> TFEYGDGI;> HHHHHHMAIYADNSYSIGNTPLVRLKHFGHNGNVVVKIEGRNPSYSVKCRIGANMVWQAEKDGTLTKGKEIVDATSGNTGIALAYVAAAR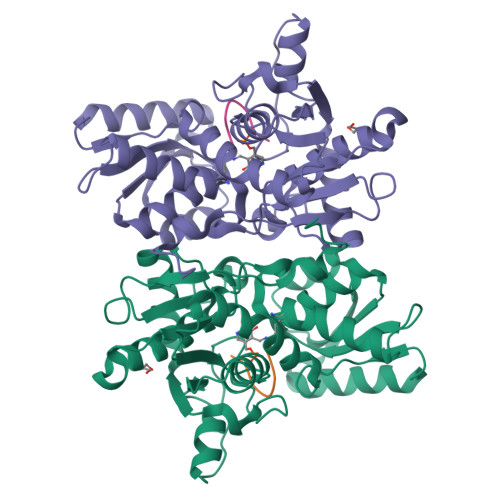GYKITLTMPETMSLERKRLLCGLGVNLVLTEGAKGMKGAIAKAEEIVASDPSRYVMLKQFENPANPQIHRETTGPEIWKDTDGKVDVVVAGVGTGGSITGISRAIKLDFGKQITSVAVEPVESPVISQTLAGEEVKPGPHKIQGIGAGFIPKNLDLSIIDRVETVDSDTALATARRLMAEEGILAGISSGAAVAAADRLAKLPEFADKLIVVILPSASERYLSTALFEGIEG> GPGSMASSSHNPVILLKRILSLTESSPFILCLDSIAQTSYKLIQEFVHQSKSKGNEYPIVYISFETVNKPSYCTQFIDATQMDFVHLVKQIISYLPAATATQAKKHMVIIDSLNY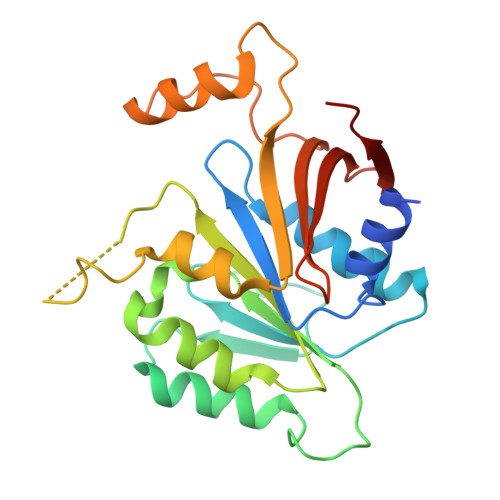ISTEYITRFLSEIASPHCTMVATYHKDIKDENRTVIPDWNNNYPDKLTLLQFMATTIVDIDVVLTGTLDTEEVSELLNEFRIPRGLNNDIFQLRLVNKRKSGRSLEYDFIVNSNTHEYELLSTTKQE> SDKLNEEAAKNIMVGNRCEVTVGAQMARRGE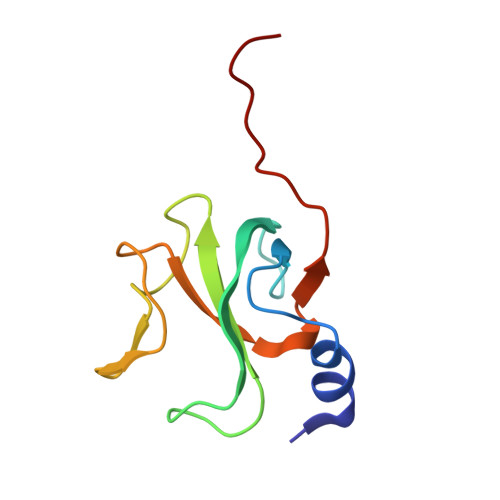VAYVGATKFKEGVWVGVKYDEPVGKNDGSVAGVRYFDCDPKYGGFVRPVDVKVGDFPELSIDEI> XXXXXXXXXXXX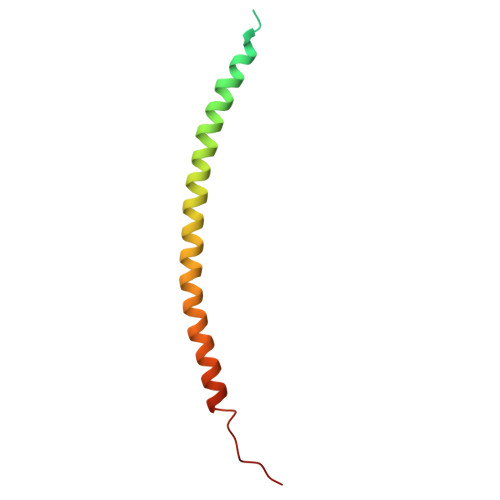XXGSHMASMTGGQQMGRGSEFARENEMDENLEQVSGIIGNLRHMALDMGNEIDTQNRQIDRIMEKADSNKTRIDEANQRATKML>[4x]MAETKEFKTLYNLFIDSYLQKLAQHSIPTNVTCAIHIGEVIGQFKNCALRITNKCMSNSRLSFTLMVESFIEVISLLPEKDRRAIAEEIGIDLDDVPSAVSKL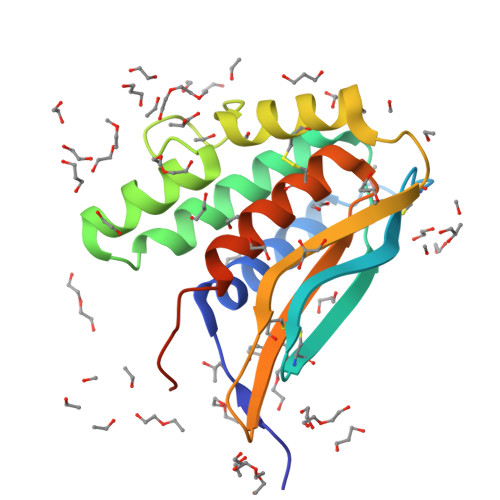EKNCNAYAEVNNIIDIQKLDIGECSAPPGQHMLLQIVNTGSAEANCGLQTIVKSLNKIYVPPIIENRLPYYDP>KFAEHLSAHITPEWRKQYIQYEAFKDMLYSAQDQAPSVEVTDEDTVKRYFAKFEEKFFQTCEKELAKINTFYSEKLAEAQRRFATLQNELQSSLDAQKESTGVTTLRQRRKPVFHLSHEERVQHRNIKDLKLAFSEFYLSLILLQNYQNLNFTGFRKILKKHDKILETSRGADWRVAHVEVAPFYTCKKINQLISETEAVVTNELEDGDRQKAMKRLRVPPLGAAQPAPAWTTFRVGLFCGIFIVLNITLVLAAVFKLETDRSIWPLIRIYRGGFLLIEFLFLLGINTYGWRQAGVNHVLIFELNPRSNLSHQHLFEIAGFLGILWCLSLLACFFAPISVIPTYVYPLALYGFMVFFLINPTKTFYYKSRFWLLKLLFRVFTAPFHKVGFADFWLADQLNSLSVILMDLEYMICFYSLELKWDESKGLLPNNSEESGICHKYTYGVRAIVQCIPAWLCFIQCLRRYRDTKRAFPHLVNAGKYSTTFFMVTFAALYSTHKERGHSDTMVFFYLWIVFYIISSCYTLIWDLKMDWGLFDKNAGENTFLREEIVYPQKAYYYCAIIEDVILRFAWTIQISITSTTLLPHSGDIIATVFAPLEVFRRFVWNFFRLENEHLNNCGEFR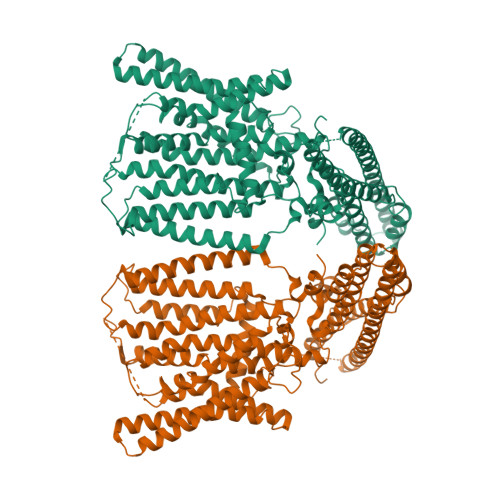AVRDISVAPL[2x]> MFSNLSKRWAQRTLSKSFYSTATGAASKSGKLTQKLVTAGVAAAGITASTLLYADSLTAEAMTAAEHGLHAPAYAWSHNGPFETFDHASIRRGYQVYREVCAACHSLDRVAWRTLVGVSHTNEEVRNMAEEFEYDDEPDEQGNPKKRPGKLSDYIPGPYPNEQAARAANQGALPPDLSLIVKARHGGCDYIFSL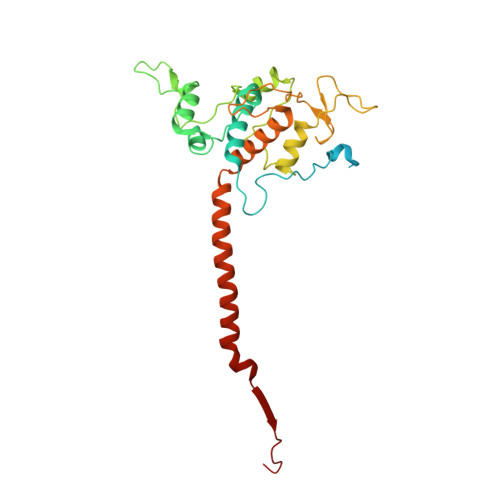LTGYPDEPPAGVALPPGSNYNPYFPGGSIAMARVLFDDMVEYEDGTPATTSQMAKDVTTFLNWCAEPEHDERKRLGLKTVIILSSLYLLSIWVKKFKWAGIKTRKFVFNPPKPRK> HHHHHHMAQDRKKVLVLGAGYAGLQTVTKLQKAISTEEAEITLINKNEYHYEATWLHEASAGTLNYEDVLYPVESVLKKDKVNFVQAEVTKIDRDAKKVETNQGIYDFDILVVALGFVSETFGIEGMKDHAFQIENVITARELSRHIEDKFANYAASKEKDDNDLSILVGGAGFTGVEFLGELTDRIPELCSKYGVD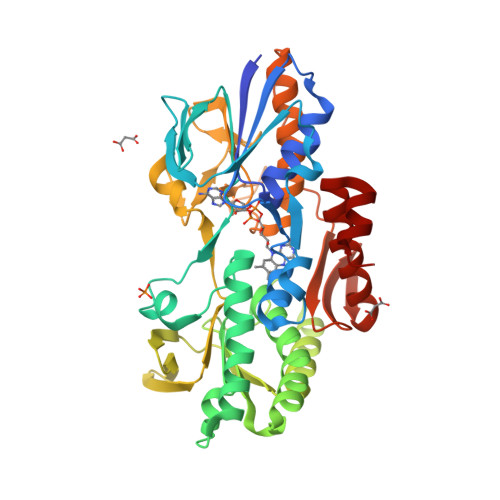QNKVKITCVEAAPKMLPMFSEELVNHAVSYLEDRGVEFKIATPIVACNEKGFVVEVDGEKQQLNAGTSVWAAGVRGSKLMEESFEGVKRGRIVTKQDLTINGYDNIFVIGDCSAFIPAGEERPLPTTAQIAMQQGESVAKNIKRILNGESTEEFEYVDRGTVCSLGSHDGVGMVFGKPIAGKKAAFMKKVIDTRAVFKIGGIGLAFKKGKF> LQAHQDIIANIGEKLGLPLTFDDNNQCLLLLDSDIFTSIEAKDDIWL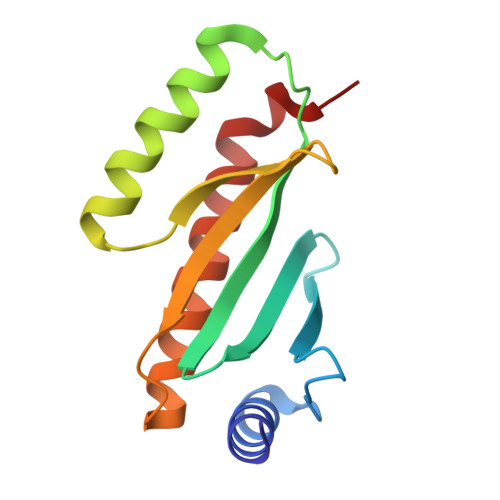LNGMIIPLSPVCGDSIWRQIMVINGELAANNEGTLAYIDAAETLLLIHAITDLTNTYHIISQLESFVNQQEALKNILQEYAKV>[4x]MNLKDKILGVAKELFIKNGYNATTTGEIVKLSESSKGNLYYHFKTKENLFLEILNIEESKWQEQWKKEQI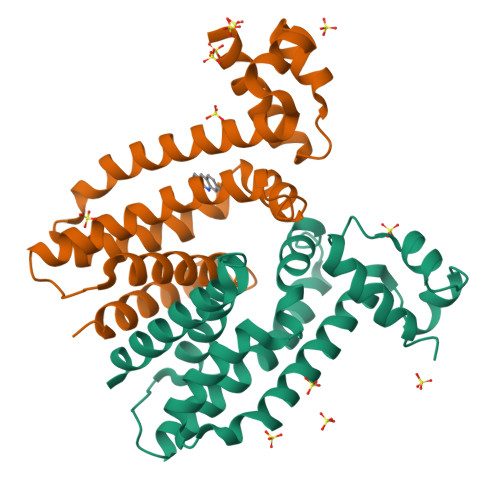KCKTNREKFYLYNELSLTTEYYYPLQNAIIEFYTEYYKTNSINEKMNKLENKYIDAYHVIFKEGNLNGEWSINDVNAVSKIAANAVNGIVTFTHEQNINERIKLMNKFSQIFLNGLSKHHHHHH>[2x]MTVSTPPSIATGNAPSPDYRVEILSESLPFIQKFRGKTIVVKYGGAAMTSPELKSSVVSDLVLLACVGLRPILVHGGGPDINRYLKQLNIPAEFRDGLRVTDATTMEIVSMVLVGKVNKNLVSLINAAGATAVGLSGHDGRLLTARPVPNSAQLGFVGEVARVDPSVLRPLVDYGYIPVIASVAADDSGQAYNINADTVAGELAAALGAEKLILLTDVAGILENKEDPSSLIKEIDIKG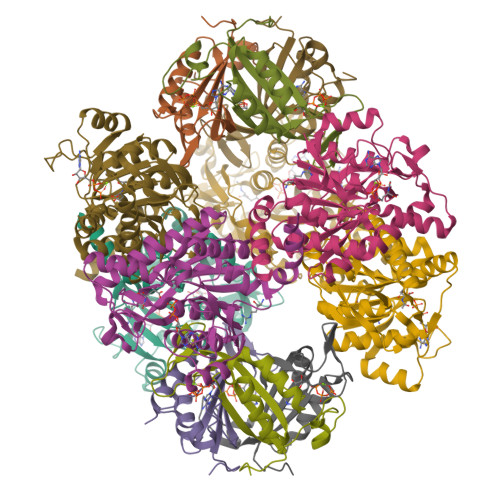VKKMIEDGKVAGGMIPKVKCCIRSLAQGVKTASIIDGRRQHSLLHEIMSDEGAGTMITG;>[2x]MQISSDYIPDSKFYKVEAIVRPWRIQQVSSALLKIGIRGVTVSDVRGFGAQGGSTERHGGSEFSEDKFVAKVKMEIVVKKDQVESVINTIIEGARTGEIGDGKIFVLPVSDVIRVRTGERGEKAEKMTGDMLSPS>[6x]GLVPRGSHMLEAQVQFASLWKRLVECINGLVNEANFDCNPGGLSVQAMDSSHVAL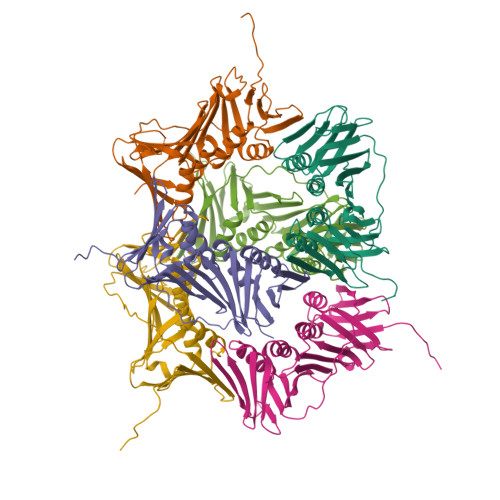VHMLLRDDCFVKYQCGRNSILGLNLASLSKVLKIVDSNDSLSLRHDDDSDVVTLTSENPEKTRKCEYQLKLLEIEAESMGIPEMDYRSTVTLNSAEFAKIVRDMQVFGDTVTIAISKEGVKFSSSGDVGQGYTFLQAAGVSDRSTKSEVKAEVKAEARDDDEEPLSRKYGKADSSANAIGVEVTMEEPITLSFALRFMGIFAKGSTLSERVTLKFAKDSPCMVEYGIDNVGYLRYYLAPKVDDAE> RLYRMYRTPDVPKGCEGPCKVQSYEQRHDISHVGKVLCVSDVTRGNGLT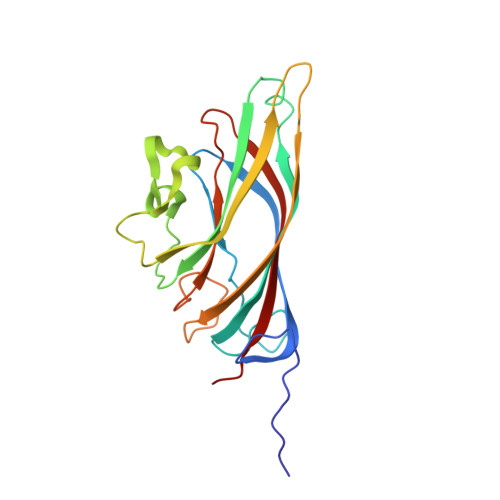HRVGKRFCVKSVYVLGKIWMDENIKTKNHTNTVMFYLVRDRRPFGTAMDFGQVFNMYDNEPSTATIKNDLRDRYQVLRKFTSTVTGGQYASKEQALVKKFMKINNYVVYNHQEAAKYDNHTENALLLYMACTHASNPVYATLKIRIYFYDSVQN> DSMYGFIGTDVVLHCSFANPLPGVKITQVTWQKATNGSKQNVAIYNPAMGVSVLAPY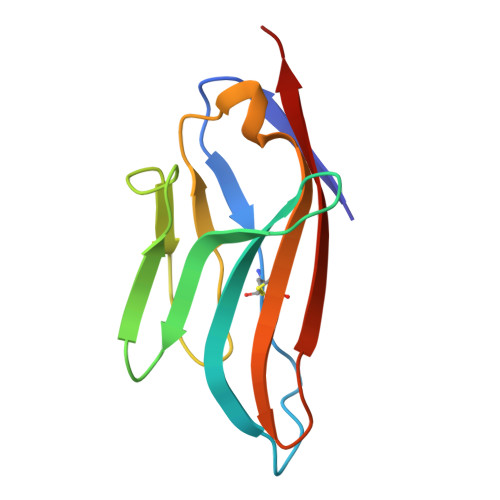RERVEFLRPSFTDGTIRLSRLELEDEGVYICEFATFPAGNRESQLNLTVMAK3-[3-(tert-butylsulfanyl)-1-[(4-chlorophenyl)methyl]-5-(propan-2-yl)-1H-indol-2-yl]-2,2-dimethylpropanoic 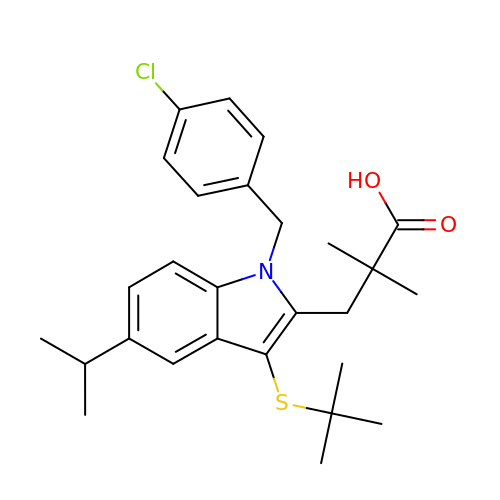acid | C27 H34 Cl N O2 S | QAOAOVKBIIKRNL-UHFFFAOYSA-N2-[(4-chlorobenzyl)amino]ethanesulfonic acid | 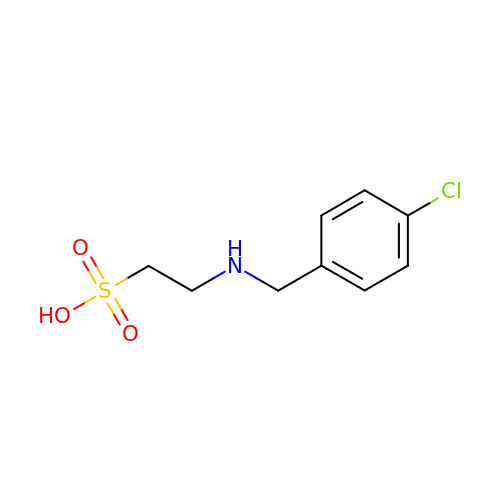C9 H12 Cl N O3 S | LPASPBAPDABFEL-UHFFFAOYSA-N> EQLTKCEVFRELKDLKGYGGVSLPEWVCTTFHTSGYDTQAIVQNNDSTEYGLFQ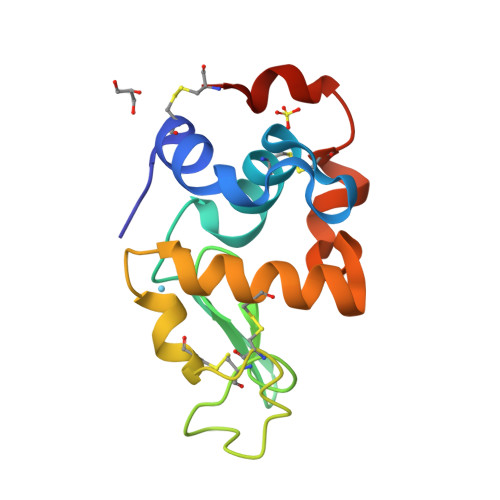INNKIWCKDDQNPHSSNICNISCDKFLDDDLTDDIMCVKKILDKVGINYWLAHKALCSEKLDQWLCEKL HPP patients exhibit hypo-mineralization and osteopenia due to the deficiency or malfunction of tissue non-specific alkaline phosphatase (TNAP), which catalyzes the hydrolysis of phosphate-containing molecules outside the cells, promoting the deposition of hydroxyapatite in the extracellular matrix. Several proteins enriched in the matrix vesicles supply sufficient phosphate for the crystallization of hydroxyapatite, and among them, the TNAP catalyzes the hydrolysis reaction using the pyrophosphate and organic phosphate esters as the substrates, such as pyrophosphate (PPi), pyridoxal phosphate (PLP) and phosphoethanolamine (PEA). The catalytic center of hTNAP is comprised of the catalytic residue S110 and three metal binding sites, one for Mg2+ and two for Zn2+ (1 and 2). The calcium-binding site includes the acidic residues E235, E291, and D306 forming strong static electric interactions with the Ca2+ ion, as well as R223, Y236, and T305 stabilizing the local conformation of the binding pocket.

Crystallization trials showed the crystals of purified hTNAP could grow in both acidic and basic pH conditions diffracting to about 5–10 Å resolution. In both structures determined with hTNAP crystals grown in acidic and basic pH conditions, four TNAP dimers, i.e., protomers A-B, C-D, E-F, and G-H, form an X-shape homo-octamer stabilized with the molecular contacts among protomers B, F, D, and H. The TNAP octamer is maintained with four major interfaces between dimeric TNAPs. Two pairs of dimers, A-B/C-D and E-F/G-H, first form two tetramers with a large interface (interface L) comprising residues from helices 1–3, 18, and 20 via a series of static electric interactions and hydrogen bonds among H79 and D25/D31, E35, and H78, K38/K45 and E311, S364-S368, and T366-T366 from the contacting protomers. The tetramers A/B/C/D and E/F/G/H then dimerize to form the octamer with two small interfaces (interface S) comprising H7, H14, and some loops. Interestingly, multiple HPP-associated mutation sites were mapped in interface L and S, including D156, K264, A492, and C497 from interface S and Y28, E311, T366, and S368 from interface L. The crystallographic analysis of hTNAP has uncovered an unexpected octameric structure that has not been observed in other previously reported AP structures. However, the disruption of the hTNAP function resulting from mutations on the octameric interface implies that hTNAP may be stabilized by octamerization, which prevents the interfaces from exposure. The conserved catalytic residue S110 was solved as the unphosphorylated form in all the protomers, which serve as a nucleophile in attacking the phosphorous. The hTNAP dimer is maintained by the static electric interactions between R71-D458, as well as the hydrogen bonds and hydrophobic interactions among residues such as T68, T85, K99, T103, Q106, H341, Y388, T389, R391, D404, N417, S445, H454, V382, L414, V447, L449, and R450.

>[8x]MKTIIALSYIFCLVFAGRALVPEKEKDPKYWRDQAQETLKYALELQKLNTNVAKNVIMFLGDGMGVSTVTAARILKGQLHHNPGEETRLEMDKFPFVALSKTYNTNAQVPDSAGTATAYLCGVKANEGTVGVSAATERSRCNTTQGNEVTSILRWAKDAGKSVGIVTTTRVNHATPSAAYAHSADRDWYSDNEMPPEALSQGCKDIAYQLMHNIRDIDVIMGGGRKYMYPKNKTDVEYESDEKARGTRLDGLDLVDTWKSFKPRYKHSHFIWNRTELLTLDPHNVDYLLGLFEPGDMQYELNRNNVTDPSLSEMVVVAIQILRKNPKGFFLLVEGGRIDHGHHEGKAKQALHEAVEMDRAIGQAGSLTSSEDTLTVVTADHSHVFTFGGYTPRGNSIFGLAPMLSDTDKKPFTAILYGNGPGYKVVGGERENVSMVDYAHNNYQAQSAVPLRHETHGGEDVAVFSKGPMAHLLHGVHEQNYVPHVMAYAACIGANLGHCAPAA> MKSKKILIVGAGFSGAVIGRQLAEKGHQVHIIDQRDHIGGNSYDARDSETNVMVHVYGPHIFHTDNETVWNYVNKHAEMMPYVNRVKATVNGQVFSLPINLHTINQFFSKTCSPDEARALIAEKGDSTIADPQTFEEEALRFIGKELYEAFFKGYTIKQWGMQPSELPASILKRLPVRFNYDDNYFNHKFQGMPKCGYTQMIKSILNHENIKVDLQREFIVEERTHYDHVFYSGPLDAFYGYQYGRLGYRTLDFKKFTYQGQYQGCAVMNYCSVDVPYTRITEHKYFSPWEQHDGSVCYKEYSRAC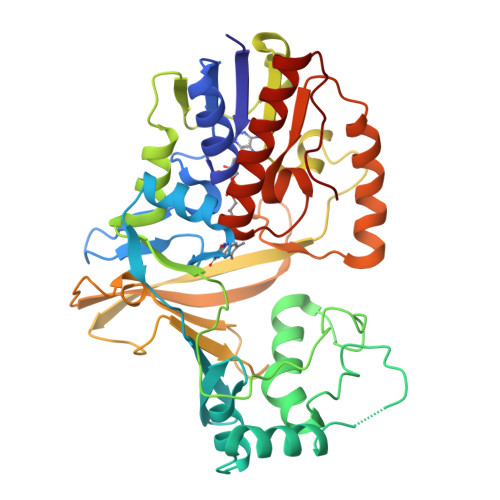EENDIPYYPIRQMGEMALLEKYLSLAENETNITFVGRLGTYRYLDMDVTIAEALKTAEVYLNSLTENQPMPVFTVSVR>MRSMKALQKALSRAGSHCGRGGWGHPSRSPLLGGGVRHHLSEAAAQGRETPHSHQPQHQDHDSSESGMLSRLGDLLFYTIAEGQERIPIHKFTTALKATGLQTSDPRLRDCMSEMHRVVQESSSGGLLDRDLFRKCVSSNIVLLTQAFRKKFVIPDFEEFTGHVDRIFEDVKELTGGKVAAYIPQLAKSNPDLWGVSLCTVDGQRHSVGHTKIPFCLQSCVKPLTYAISISTLGTDYVHKFVGKEPSGLRYNKLSLNEEGIPHNPMVNAGAIVVSSLIKMDCNKAEKFDFVLQYLNKMAGNEYMGFSNATFQSEKETGDRNYAIGYYLKEKKCFPKGVDMMAALDLYFQLCSVEVTCESGSVMAATLANGGICPITGESVLSAEAVRNTLSLMHSCGMYDFSGQFAFHVGLPAKSAVSGAILLVVPNVMGMMCLSPPLDKLGNSHRGTSFCQKLVSLFNFHNYDNLRHCARKLDPRREGAEIRNKTVVNLLFAAYSGDVSALRRFALSAMDMEQKDYDSRTALHVAAAEGHIEVVKFLIEACKVNPFAKDRW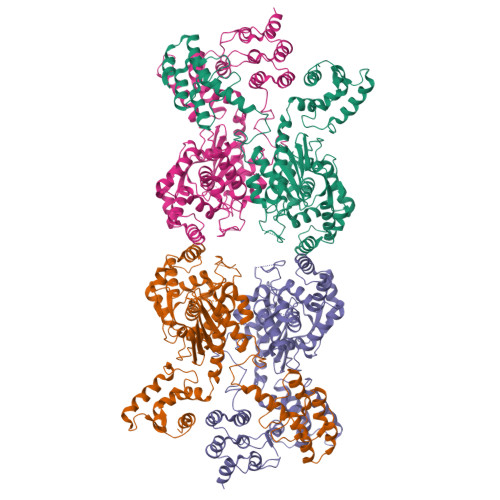GNIPLDDAVQFNHLEVVKLLQDYQDSYTLSETQAEAAAEALSKENLESMV[4x]>[2x]RKILIIEDSELQRKLLSRWVSKNGYIAIEAESISVAREKIISESIDVVLLDWELPDGNGIDLISDILSTSPVGWLPIIMVTGHTEPEYFKIAIEAGATDYITKPAKEIELLARIFSALRIKALHDQLRETAIRDVMTGLYNRRYMEERIEQEFQRCKRHDSLLSMAMIDIDKFKNINDTYGHEIGDQVIKQLAHELKTSFAKSAIISRFGGEEFVILFPETGVVDATRI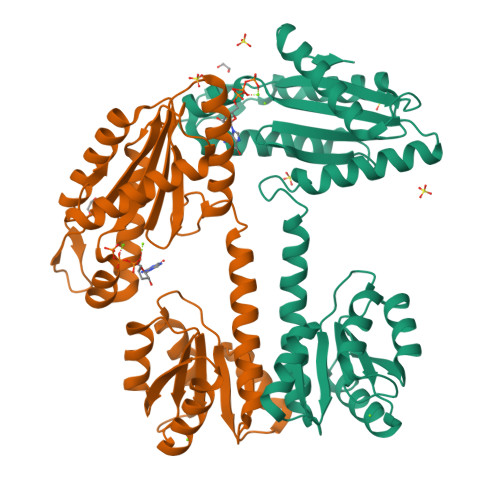LDRVRENVSKLEMKSDTDQIFHFTFSGGVAGGDLSDIQSNQELLKIADKNLYEAKSSGRNQIIS> QDNSRYTHFLTQHYDAKPQGRDDRYCE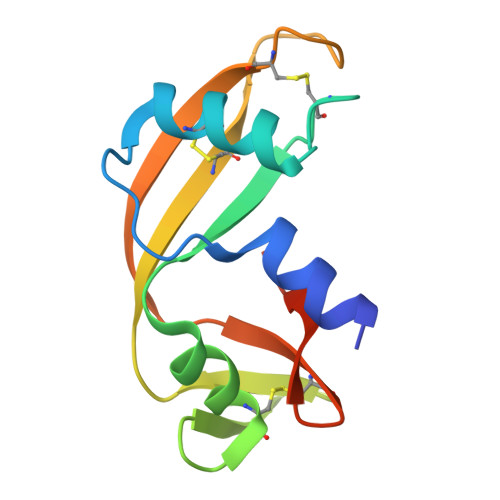SIMRRRGLTSPCKDINDFIHGNKRSIKAICENKNGNPHRENLRISKSSFQVTTCKLHGGSPWPPCQYRATAGFRNVVVACENGLPVHLDQSIFRRP> MAPVQGSYDYDLIVIGGGSAGLACAKEAVLNGARVACLDFVKPTPTLGTKWGVGGTCVNVGCIPKKLMHQASLLGEAVHEAAAYGWNVDDKIKPDWHKLVQSVQNHIKSVNWVTRVDLRDKKVEYINGLGSFVDSHTLLAKLKSGERTITAQTFVIAVGGRPRYPDIPGAVEYGITSDDLFSLDREPGKTLVVGAGYIGLECAGFLKGLGYEPTVMVRSIVLRGFDQQMAELVAASMEERGIPFLRKTVPLSVEKQDDGKLLVKYKNVETGEESEDVYDTVLWAIGRKGLVDDLNLPNAGVTVQKDKIPVDSQEATNVANIYAVGDIIYGKPELTPVAVLAGRLLARRLYGGSTQRMDYKDVATTVFTPLEYACVGLSEEDAVKQFGADEIEVFHGYYKPTEFFIPQKSVRYCYLKAVAERHGDQRVYGLHYIGPV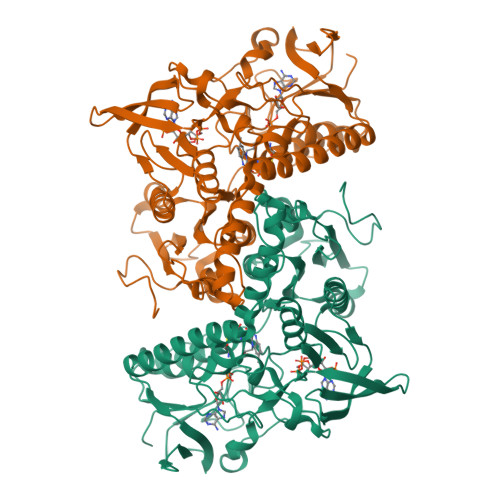AGEVIQGFAAALKSGLTINTLINTVGIHPTTAEEFTRLAITKRSGLDPTPAS FORMANILIDE | C7 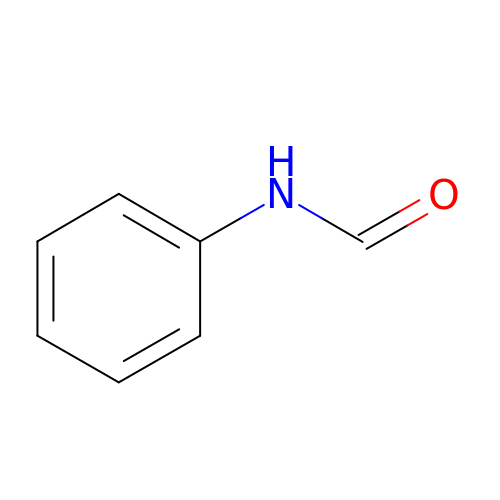H7 N O | DYDNPESBYVVLBO-UHFFFAOYSA-N>[3x]ATAAEIAALPRQKVELVDPPFVHAHSQVAEGGPKVVEFTMVIEEKKIVIDDAGTEVHAMAFNGTVPGPLMVVHQDDYLELTLINPETNTLMHNIDFHAATGALGGGGLTEINPGEKTILRFKATKPGVFVYHCAPPGMVPWHVVSGGNG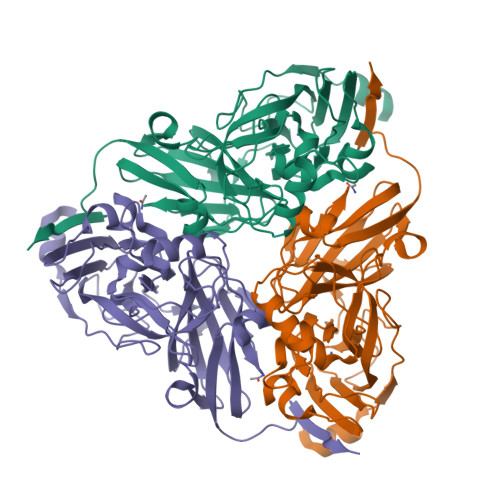AIMVLPREGLHDGKGKALTYDKIYYVGEQDFYVPRDENGKYKKYEAPGDAYEDTVKVMRTLTPTHVVFNGAVGALTGDKAMTAAVGEKVLIVHSQANRDTRPHLIGGHGDYVWATGKFNTPPDVDQETWFIPGGAAGAAFYTFQQPGIYAYVNHNLIEAFELGAAAHFKVTGEWNDDLMTSVLAPSG> MEPLYDKNGAVLFGEPSDTHPQSTLKLPHPRGEKEVIVGIRDLPRKGDCRTGNRLGPVSGLFVKPGPVFYQDYSGPVYHRAPLEQFKQAPMCEVTKRIGRVTGSDGNLYHMYVCTDGCILVKTAKREGQDVLKWVYNVLDSPIWVTS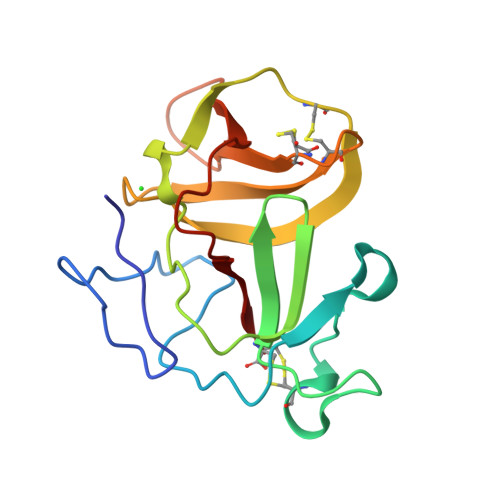C> MNSSSFPYFISPEQAMRERSELARKGIARAKSVVALAYAGGVLFVAENPSRSLQKISELYDRVGFAAAGKFNEFDNLRRGGIQFADTRGYAYDRRDVTGRQLANVYAQTLGTIFTEQAKPYEVELCVAEVAHYGETKRPELYRITYDGSIADEPHFVVMGGTTEPIANALKESYAENASLTDALRIA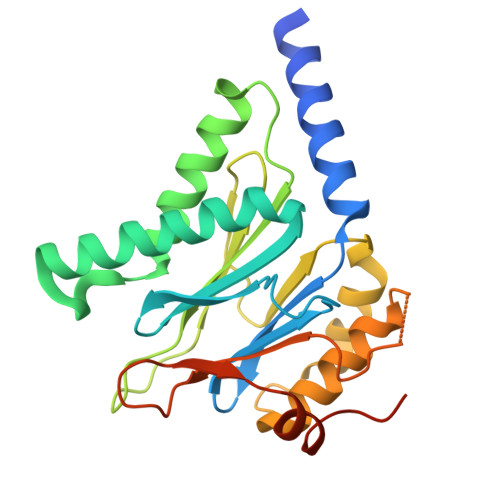VAALRAGSADTSGGDQPTLGVASLEVAVLDANRPRRAFRRITGSALQALLVDQESPQSDGESSG> NLSEL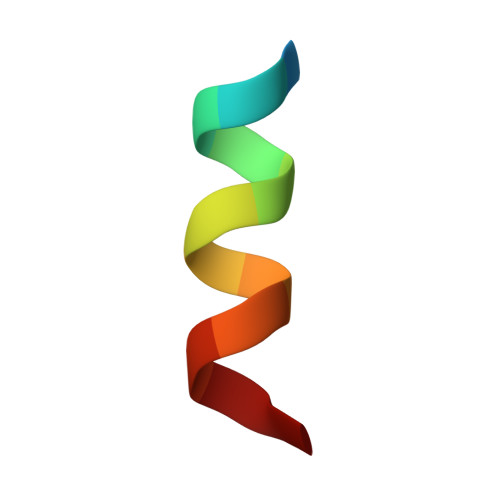DRLLLELN>[2x]GPHMVVAGIDPGITHLGLGVVAVEGKGALKARLLHGEVVKTSPQEPAKERVGRIHARVLEVLHRFRPEAVAVQEQFFYRQNELAYKVGWALGAVLVAAFEAGVPVYAYGPMQVKQALAGHGHAAKEEVALMVRGILGLKEAPRPSHLADALAIALTHAFYARMGTAKPL

RuvC resolvase from Gram-negative bacteria belongs to the retroviral integrase superfamily with a characteristic RNase H fold. RuvC is a dimeric endonuclease that requires divalent metal ions for activity. RuvC resolves HJs by symmetrically cleaving two of its DNA strands. Substrate binding does not depend on the DNA sequence, but the cleavage is specific and occurs preferentially at the (A/T)TT↓(G/C) cognate sequence.

Here, we present the crystal structure of T. thermophilus RuvC in complex with a short synthetic HJ solved at 3.75 Å resolution. To inhibit HJ cleavage during crystallization, we also prepared an inactive Tt-RuvC variant with E70Q substitution at the active site. The junction in complex with RuvC has the same non-crystallographic 2-fold symmetry as the protein dimer. The structure of the DNA can be described as tetrahedral. The arms are unstacked, and the two opposite arms located in the vicinity of the active sites are pointing downward from the plane between the HJ exchange point and the protein. RuvC approaches the scissile phosphates from the minor groove side of the double helix. The protein covers 4 bp on arms 1 and 2 and 8 bp on arms 3 and 4, which is consistent with footprinting data. The exchange point of the junction is stabilized by the N-termini of helices B from each subunit, which also participate in dimer formation. However, in our complex structure, the loops from both dimer subunits adopt a similar conformation, suggesting that a different mechanism is responsible for sequential cleavages by RuvC.>[2x]XLA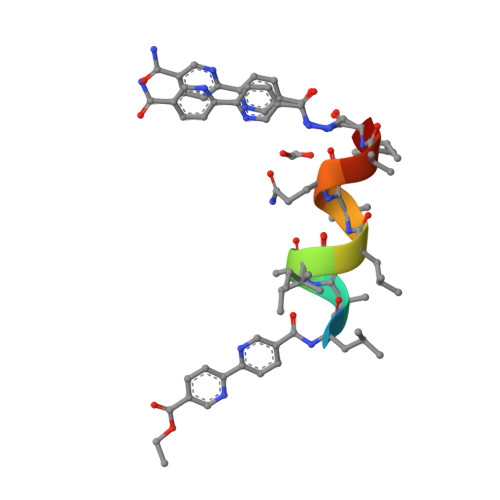AILAQALX2-[2-[carboxymethyl(phenylmethyl)amino]ethyl-[(2-hydroxyphenyl)methyl]amino]ethanoic 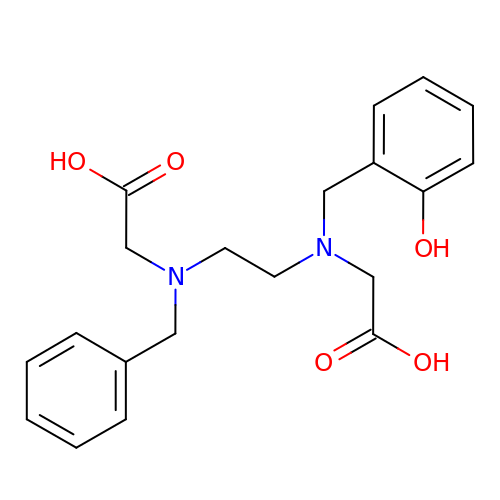acid | C20 H24 N2 O5 | JSDNXVMPVNBNSK-UHFFFAOYSA-N>[2x]MAASATAAAVAAEVISVHS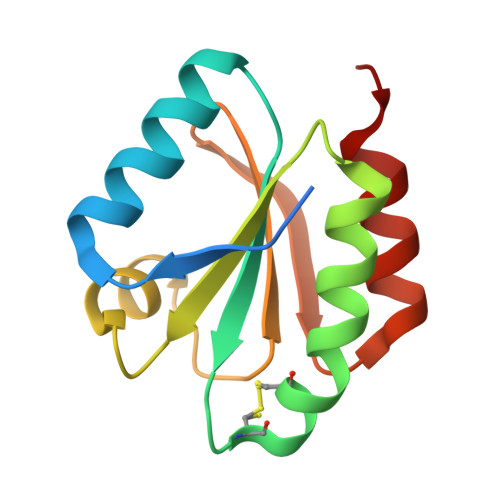LEQWTMQIEEANTAKKLVVIDFTASWCGPCRIMAPVFADLAKKFPNAVFLKVDVDELKPIAEQFSVEAMPTFLFMKEGDVKDRVVGAIKEELTAKVGLHAAAQ> MATKEQIVEHRESEIPIASQWKATFPVDLEIEKNSEMFALRYIKCASAFILDRRGILDE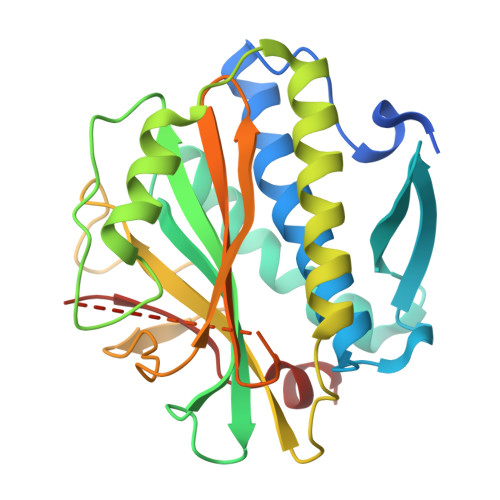KCFKTRTIDKLLVTAFQSSVPAAKRVSSTFDGLRDAIQQGYLREFAIVFYKKPNEEDINEVFAFRFAYGDEGEIFVSLNNGIDTNESSQELLQAKFVDTDNTKQMFASTIKKLHRCIKKMEPLPQGSDASFRVSYTEKAPKDYTPEGYLLSPMFYTLNQDIRKASIGIVCGGHHKIQMLAASQYLKQDFDLDKTTTLNPNMSIMANQSKRKGRISRDRHYGRVSSILDVAGSKD> MPRVRPLGPNPQDRPNWDSMNEGQRRYAMEQWNLARVRRGEYFDPPGDDDLPLTQADAIDNFDLDLLGSPQEAEQPSQQSEDGVDDFLQQVRDRQDLR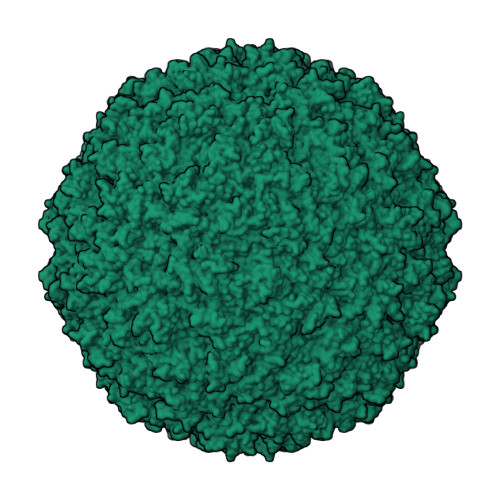DAGPSNAPQPNMADIEMSQVSSSSGGSKRGSGGGGPPSKVSKSGTSLPGTGGNLDGMVRGGSGEGGATAILRPIGLHVEKFQQTYRKKWRFLTSANANVILAEAASGERPARWALTTGMASIPWEYLFFYMSPAEYNRMKNYPGTFAKSASVRIRTWNTRVAFQTGDTQTANATLNQNKFLQVAKGIRSIPFICSTNRKYTYSDTEPMQPTGFATLTSYEYRDGLKTAMYGYDNDNKDFAKKPPADATGAEIYLQDYLTIYTNDARATTGTKILAGFPPYKNFIEEFDASACINTDVVAMDYDFSYAPLVPQFAPVPNNLITQNYNGSYPAGTKNEVTAAKTTDSSQATAPTQVRNAPRKYIQGPHADTTFFDEEQNYLRVPIEQGGIFEEVNVETVHDTQMPSINVGIRAVPKLTTIDETTQANSWLDAQGYFEVDCVLTTESVDPYTYIKGGCYSANTKSQLQYFASDGRPIAKVYDNPNVYGRMQMIKTVKP>[2x]GMKFSKFGQKFTQPTGISQLMDDLGDALKSDQPVNMLGGGNPAKIDAVNELFLETYKALGNDNDTGKANSSAIISMANYSNPQGDSAFIDALVGFFNRHYDWNLTSENIALTNGSQNAFFYLFNLFGGAFVNEHSQDKESKSVDKSILLPLTPEYIGYSDVHVEGQHFAAVLPHIDEVTHDGEEGFFKYRVDFEALENLPALKEGRIGAICCSRPTNPTGNVLTDEEMAHLAEIAKRYDIPLI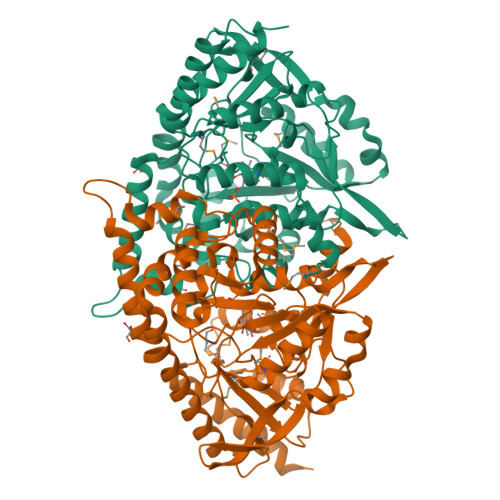IDNAYGMPFPNIIYSDAHLNWDNNTILCFSLSKIGLPGMRTGIIVADAKVIEAVSAMNAVVNLAPTRFGAAIATPLVANDRIKQLSDNEIKPFYQKQATLAVKLLKQALGDYPLMIHKPEGAIFLWLWFKDLPISTLDLYERLKAKGTLIVPSEYFFPGVDVSDYQHAHECIRMSIAADEQTLIDGIKVIGEVVRELYDNK>MPSFNPVRFLELPIDIRKEVYFHLDGNFCGAHPYPIDILYKSNDVELPGKPSYKRSKRSKKLLRYMYPVFATYLNIFEYSPQLIEKWLEYAFWLRYDCLVLDCFKVNHLYDGTLIDALEWTYLDNELRLAYFNKASMLEVWYTFKEYKKWVIDSVAFDELDLLNVSNIQFNIDNLTPQLVDKCLSILEQKDLFATIGEVQFGQDEEVGEEKDVDVSGANSDENSSPSSTIKNKKRSASKRSHSDNGNVGATHNQLTSISVIRTIRSMESMKSLRKITVRGEKLYELLINFHGFRDNPGKTISYIVKRRINEIRLSRMNQISRTGLADFTRWDNLQKLVLSRVAYIDLNSIVFPKNFKSLTMKRVSKIKWWNIEENILKELKVDKRTFKSLYIKEDDSKFTKFFNLRHTRIKELDKSEINQITYLRCQAIVWLSFRTLNHIKLQNVSEVFNNIIVPRALFDSKRVEIYRCEKISQVLVI[2x];>MFNRTTQLKSKHPCSVCTRRKVKCDRMIPCGNCRKRGQDSECMKSTKLITASSSKEYLPDLLLFWQNYEYWITNIGLYKTKQRDLTRTPANLDTDTEECMFWMNYLQKDQSFQLMNFAMENLGALYFGSIGDISELYLRVEQYWDRRADKNHSVD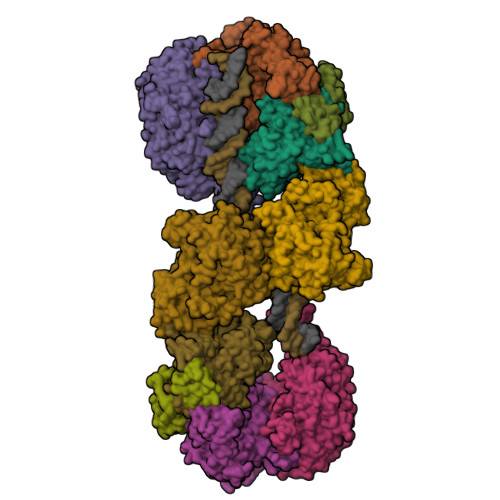GKYWDALIWSVFTMCIYYMPVEKLAEIFSVYPLHEYLGSNKRLNWEDGMQLVMCQNFARCSLFQLKQCDFMAHPDIRLVQAYLILATTTFPYDEPLLANSLLTQCIHTFKNFHVDDFRPLLNDDPVESIAKVTLGRIFYRLCGCDYLQSGPRKPIALHTEVSSLLQHAAYLQDLPNVDVYREENSTEVLYWKIISLDRDLDQYLNKSSKPPLKTLDAIRRELDIFQYKVDSLEEDFRSNNSRFQKFIALFQISTVSWKLFKMYLIYYDTADSLLKVIHYSKVIISLIVNNFHAKSEFFNRHPMVMQTITRVVSFISFYQIFVESAAVKQLLVDLTELTANLPTIFGSKLDKLVYLTERLSKLKLLWDKVQLLDSGDSFYHPVFKILQNDIKIIELKNDEMFSLIKGLGSLVPLNKLRQESLLEEEDENNTEPSDFRTIVEEFQSEYNISDILS[4x];>[2x]MVTSNVVLVSGEGERFTVDKKIAERSLLLKNYLNDMHDSNLQNNSDSESDSDSETNHKSKDNNNGDDDDEDDDEIVMPVPNVRSSVLQKVIEWAEHHRDSNFPDEDDDDSRKSAPVDSWDREFLKVDQEMLYEIILAANYLNIKPLLDAGCKVVAEMIRGRSPEEIRRTFNIVNDFTPEEEAAIRRENEWAEDR;>[2x]MRSSILFLLKLMKIMDVQQQQEAMSSEDRFQELVDSLKPRTAHQYKTYYTKYIQWCQLNQIIPTPEDNSVNSVPYKDLPISAELIHWFLLDTLITDDKPGEKREETEDLDEEEENSFKIATLKKIIGSLNFLSKLCKVHENPNANIDTKYLESVTKLHTHWIDSQKAITTNETNNTNTQVLCPPLLKVSLNLWNPETNHLSEKFFKTCSEKLRFLVDFQLRSYLNLSFEERSKIRFGSLKLGKRDRDAIIYHKVTHSAEKKDTPGHHQLLALLPQDCPFICPQTTLAAYLYLRFYGIPSVSKGDGFPNLNADENGSLLQDIPILRGKSLTTYPREETFSNYYTTVFRYCHLPYKRREYFNKCNLVYPTWDEDTFRTFFNEENHGNWLEQPEAFAFPDKIPFDFKKIMNFKSPYTSYSTNAKKDPFPPPKDLLVQIFPEIDEYKRHDYEGLSQNSRDFLDLMEVLRERFLSNLPWIYKFFPNHDIFQDPIFGNSDFQSYFNDKTIHSKGSPILSFDILPGFNKIYKNKTNFYSLLIERPSQLTFASSHNPDTHPTQKQESEGPLQMSQLDTTQLNELLKQQSFEYVQFQTLSNFQILLSVFNKIFEKLEMKKSSRGYILHQLNLFKITLDERIKKSKIDDADKFIRDNQPIKKEENIVNEDGPNTSRRTKRPKQIRLLSIADSSDESSTEDSNVFKKDGESIEDGAYGENEDENDSEMQEQLKSMINELINSKISTFLRDQMDQFELKINALLDKILEEKVTRIIEQKLGSHTGKFSTLKRPQLYMTEEHNVGFDMEVPKKLRTSGKYAETVKDNDDHQAMSTTASPSPEQDQEAKSYTDEQEFMLDKSIDSIEGIILEWFTPNAKYANQCVHSMNKSGNKSWRANCEALYKERKSIVEFYIYLVNHESLDRYKAVDICEKLRDQNEGSFSRLAKFLRKWRHDHQNSFDGLLVYLSN> GSGSWQTYVDDHLMCDIEGTGQHLTSAAIFGTDGTVWAKSASFPEFKPNEIDAIIKEFNEAGQLAPTGLFLGGAKYMV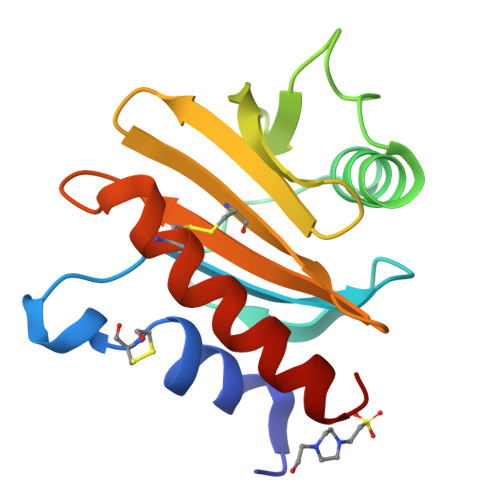IQGEAGAVIRGKKGAGGICIKKTGQAMVFGIYDEPVAPGQCNMVVERLGDYLLDQGM>MEVDPRLYFENRSKFIQDQKDKGINPYPHKFERTISIPEFIEKYKDLGNGEHLEDTILNITGRIMRVSASGQKLRFFDLVGDGEKIQVLANYSFHNHEKGNFAECYDKIRRGDIVGIVGFPGKSKKGELSIFPKETILLSACLHMLPMKYGLKDTEIRYRQRYLDLLINESSRHTFVTRTKIINFLRNFLNERGFFEVETPMMNLIAGGANARPFITHHNDLDLDLYLRIATELPLKMLIVGGIDKVYEIGKVFRNEGIDNTHNPEFTSCEFYWAYADYNDLIKWSEDFFSQLVYHLFGTYKISYNKDGPENQPIEIDFTPPYPKVSIVEEIEKVTNTILEQPFDSNETIEKMINIIKEHKIELPNPPTAAKLLDQLASHFIENKYNDKPFFIVEHPQIMSPLAKYHRTKPGLTERLEMFICGKEVLNAYTELNDPFKQKECFKLQQKDREKGDTEAAQLDSAFCTSLEYGLPPTGGLGLGIDRITMFLTNKNSIKDVILFPTMRPANGGHHHHHH[2x]

Aminoacyl-tRNA synthetases (aaRSs) catalyze the synthesis of aminoacyl-tRNAs, which are crucial building blocks for protein biosynthesis. Lysyl-tRNA synthetase (LysRS) has been validated as a promising target for antimalarial, anti-Cryptosporidium, anti-Pseudomonas aeruginosa, and anti-Mycobacterium tuberculosis therapies. The ATP-binding pocket is the most promising area for the development of LysRS inhibitors. We determined five cocrystal structures of LysRS in complex with the compounds in order to provide a basis for further optimization.

Compared to compound 36, the methoxy group in the amino meta position of compound 34 is replaced by a methoxycarbonyl group, and the substitution position of methoxy group in compound 35 is different. As a result, the ΔTm values of PfLysRS caused by compound 34 and 35 were both lower than that caused by compound 36, and the potency of compound 34 against PfLysRS was weaker than that of compound 36. To understand how these compounds are recognized by PfLysRS, we determined the cocrystal structures of PfLysRS with the compounds 34, 35, 36, and 38. Most of the interactions between the compounds and the protein were preserved compared to PfLysRS-ASP3026. The methoxy group inherited from ASP3026 in these compounds were all bound to the hydrophobic cavity formed by Arg330, Glu332, His338, Asn339, and Pro340 like ASP3026. Similarly, the carbonyl oxygen of compound 34 also formed a new H-bond with Arg330. Among these compounds, compounds 34, 36 and 38 demonstrated greater inhibitory activity on parasite growth compared to ASP3026.>PAIDYKTAFHLAPIGLVLSRDRVIEDCNDELAAIFRCARADLIGRSFEVLYPSSDEFERIGERISPVMIAHGSYADDRIMKRAGGELFWCHVTGRALDRTAPLAAGVWTFEDLSATR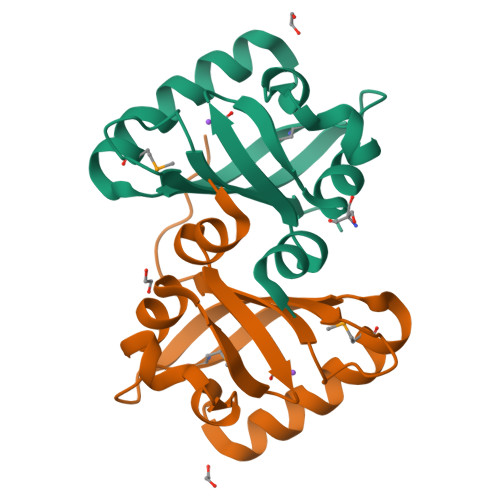RVA[2x]> GAHMSYSYDAPSDFINFSSKQKNEESKKRQWALEDFEIGRPLGKGKFGNVYLAREKQSKFILALKVLFKAQLEKAGVEHQLRREVEIQSHLRHPNILRLYGYFHDATRVYLILEYAPLGTVYRELQKLSKFDEQRTATYITELANALSYVHSKRVIHRDIKPENLLLGSAGELKIADFGW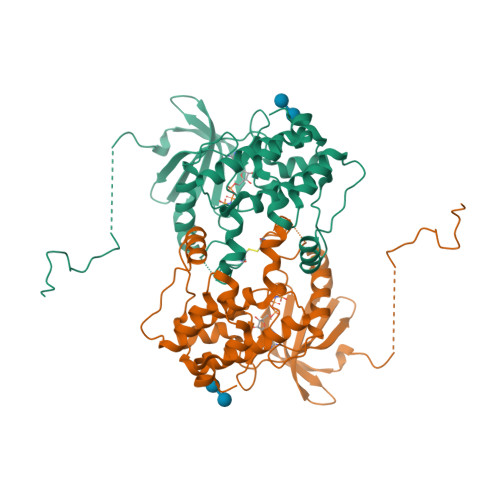SVHAPSSRRTTLCGTLDYLPPEMIEGRMHDEKVDLWSLGVLVYEFLVGKPPFEANTYQETYKRISRVEFTFPDFVTEGARDLISRLLKHNPSQRPMLREVLEHPWITANSSK4-bromo-N'-(3,4-dihydro-2H-pyrrol-5-yl)benzohydrazide 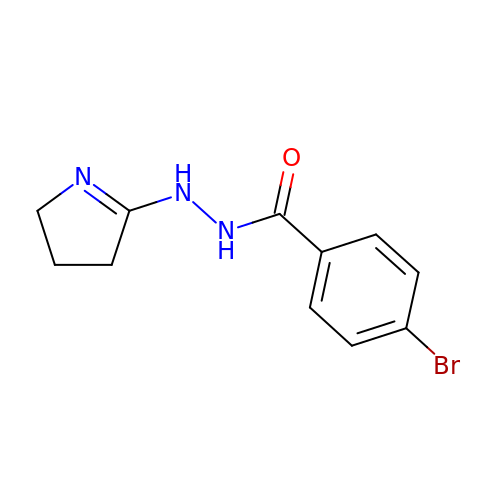| C11 H12 Br N3 O | QKAHAXIACNFPOK-UHFFFAOYSA-N>[4x]HHHHHHHVTQSSSAITPGQTAELYPGDIKSVLLTAEQIQARIAELGEQIGNDYRELSATTGQDLL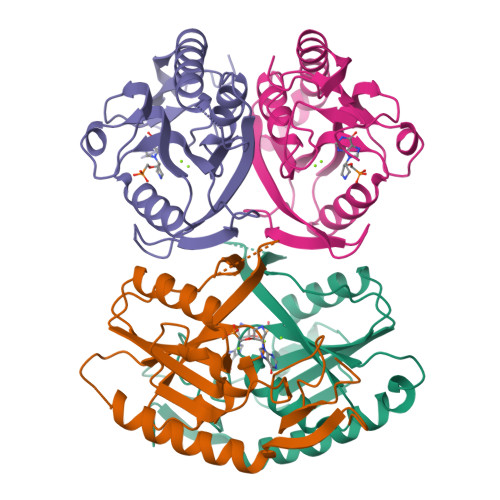LITVLKGAVLFVTDLARAIPVPTQFEFMAVSSYGSSTSSSGVVRILKDLDRDIHGRDVLIVEDVVDSGLTLSWLSRNLTSRNPRSLRVCTLLRKPDAVHANVEIAYVGFDIPNDFVVGYGLDYDERYRDLSYIGTLDPRVYQ>[2x]AANRELQASLNLLQEDQNAGRQVQMNMLPVTPWSIEGLEFSHRIIPSLYLSGDFVDYFRVDERRV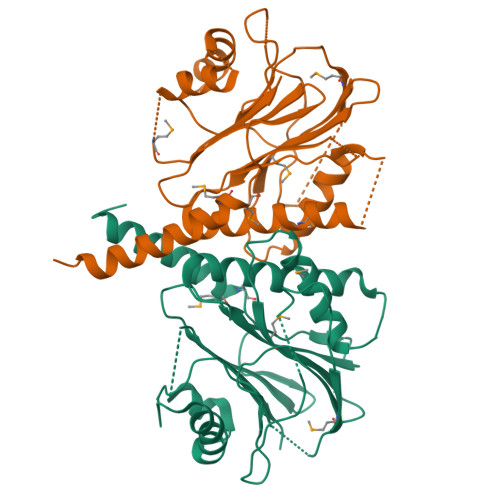AFYLADVSGHGASSAFVTVLLKFMTTRLLYESRRNGTLPEFKPSEVLAHINRGLINTKLGKHVTMLGGVIDLEKNSLTYSIGGHLPLPVLFVEGQAGYLEGRGLPVGLFDDATYDDRVMELPPSFSLSLFSDGILDVLPGATLKEKEASLPEQVAAAGGTLDGLRQVFGLANLAEMPDDIALLVLSRNLA> MVVSEVDIAKADPAAASHPLLLNGDATVAQKNPGSVAENNLCSQYEEKVRPCIDLIDSLRALGVEQDLALPAIAVIGDQSSGKSSVLEALSGVALPRGSGIVTRCPLVLKLKK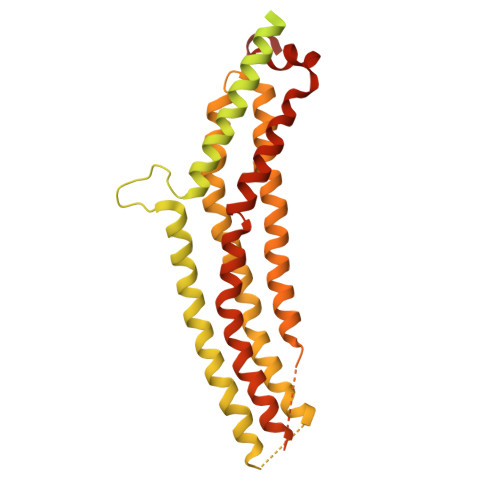LVNEDKWRGKVSYQDYEIEISDASEVEKEINKAQNAIAGEGMGISHELITLEISSRDVPDLTLIDLPGITRVAVGNQPADIGYKIKTLIKKYIQRQETISLVVVPSNVDIATTEALSMAQEVDPEGDRTIGILTKPDLVDKGTEDKVVDVVRNLVFHLKKGYMIVKCRGQQEIQDQLSLSEALQREKIFFENHPYFRDLLEEGKATVPCLAEKLTSELITHICKSLPLLENQIKETHQRITEELQKYGVDIPEDENEKMFFLIDKVNAFNQDITALMQGEETVGEEDIRLFTRLRHEFHKWSTIIENNFQEGHKILSRKIQKFENQYRGRELPGFVNYRTFETIVKQQIKALEEPAVDMLHTVTDMVRLAFTDVSIKNFEEFFNLHRTAKSKIEDIRAEQEREGEKLIRLHFQMEQIVYCQDQVYRGALQKVREKELEEEKKKKSWDFGAFQSSSATDSSMEEIFQHLMAYHQEASKRISSHIPLIIQFFMLQTYGQQLQKAMLQLLQDKDTYSWLLKERSDTSDKRKFLKERLARLTQARRRLAQFPG> GCRLCR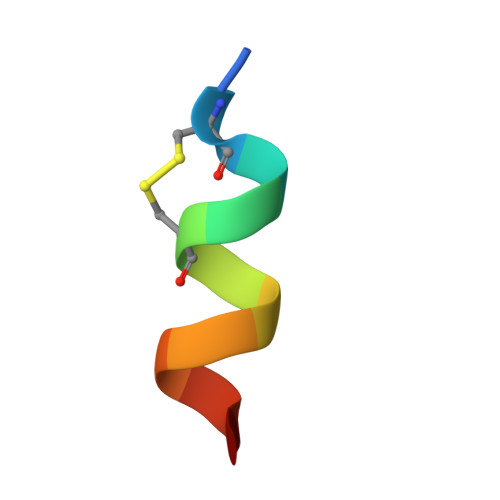LLSYAX>SMGGTHIDLLFHPPRAHLLTIKETIRKMIKEARKVIALVMDIFTDVDIFKEIVEASTRGVSVYILLDESNFNHFLNMTEKQGCSVQRLRNIRVRTVKGQDYLSKTGAKFHGKMEQKFLLVDCQKVMYGSYSYMWS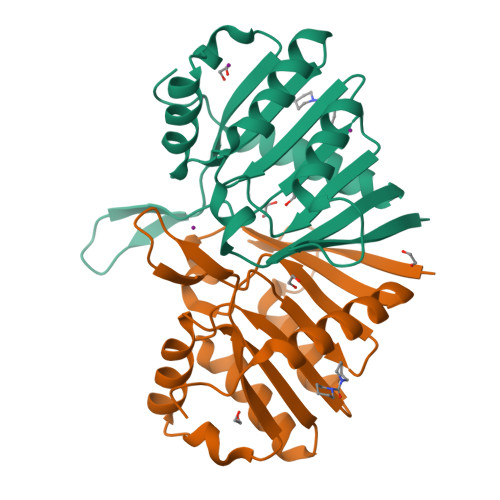FEKAHLSMVQIITGQLVESFDEEFRTLYARSCVPSSFAQEESARV[2x]>MIKKAVLPVAGLGTRFLPASKSIPKEMVTVVDRPAIEYVVREAVEAGIEQIILVTHSSKASIENYFDRNFELETTLE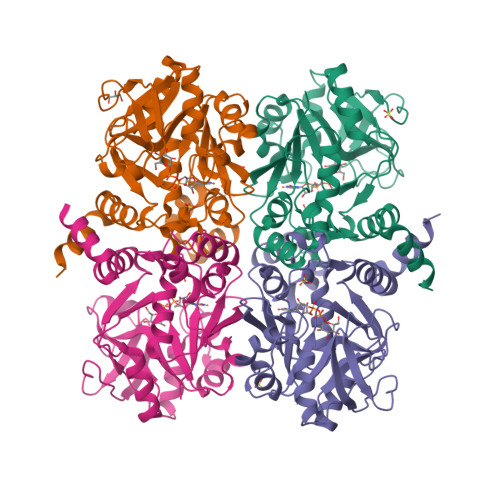QKKKFDLLAEITQIVPEHVSVISVRQPQPLGLGHAVLCAKSVVGEDDFAVLLPDVLVKDGSGQNDLSRMISRYNSSQAAQIMVEAVPDHLVDQYGIVDVAQSPNEGESIAMQGIVEKPPVGAAPSNLSVVGRYVLPAKIMQLLENTPKGAGNEIQLTDAIAMLQDTDTVEAYRMQGQTFDCGSKLGYLKAVLHYGLEHPKLGMEFKQLILELK[4x]We have previously demonstrated that Fam20A lacks an essential residue for catalysis and is therefore the first pseudokinase identified in the secretory pathway. Fam20A forms a functional complex with Fam20C and allosterically increases Fam20C activity towards secretory substrates, including the enamel matrix proteins, whose phosphorylation is critical for enamel formation. Furthermore, Fam20A binds ATP despite being catalytically inactive, the structural basis and functional impact of which remain elusive. Here, we report the nucleotide-free and ATP-bound crystal structures of Fam20A.

We determined the crystal structure of human Fam20A at 2.5 Å resolution. The kinase core of Fam20A (residues 160–525) is structurally similar to that of ceFam20, and can be superimposed onto ceFam20 with a rmsd (root-mean-square difference) of 2.1 Å over 322 aligned Cα atoms. An insertion of seventeen residues specifically exists in the Kβ1-Kβ2 loop of Fam20A. This insertion forms two short α-helices (Kα2A, Kα2B) and forces an upswing of the Kβ1-Kβ2 loop. The Kβ1-Kβ2 loop in turn levers up the Kβ6-Kβ7 loop and induces the formation of a short helix (Kα5A) in this region. Gln258Fam20A, which replaces a Glu essential for the catalytic activity of Fam20C (Glu213ceFam20), resides at the C-terminal end of the Kβ3-Kα3 loop. As a result of the upswing of this loop, Gln258Fam20A is dislodged from the ‘active site’ of Fam20A. Instead, Cys209Fam20A and Cys211Fam20A in the Kβ1-Kβ2 loop form two disulfide bonds with Cys319Fam20A and Cys323Fam20A (the two Cys that align with Cys273ceFam20 and Cys277ceFam20), respectively. These two disulfide bonds tether the Kβ1-Kβ2 loop to the Kβ6-Kβ7 loop, imposing a strong restraint on the structural flexibility of this region. In the crystal, Fam20A forms a symmetrical, face-to-face dimer.

>SSKLQALFAHPLYNVPEEPPLLGAEDSLLASQEALRYYRRKVARWNRRHKMYREQMNLTSLDPPLQLRLEASWVQFHLGINRHGLYSRSSPVVSKLLQDMRHFPTISADYSQDEKALLGACDCTQIVKPSGVHLKLVLRFSDFGKAMFKPMRQQRDEETPVDFFYFIDFQRHNAEIAAFHLDRILDFRRVPPTVGRIVNVTKEILEVTKNEILQSVFFVSPASNVCFFAKCPYMCKTEYAVCGKPHLLEGSLSAFLPSLNLAPRLSVPNPWIRSYTLAGKEEWEVNPLYCDTVKQIYPYNNSQRLLNVIDMAIFDFLIGNMDRHHYEMFTKFGDDGFLIHLDNARGFGRHSHDEISILSPLSQCCMIKKKTLLHLQLLAQADYRLSDVMRESLLEDQLSPVLTEPHLLALDRRLQTILRTVEGCIVAHGQQSVIVDGP[2x]> DNGGYVPAVVIGTGYGAAVSALRLGEAGVQTLMLEMGQLWNQPGPDGNIFCGMLNPDKRSSWFKNRTEAPLGSFLWLDVVNRNIDPYAGVLDRVNYDQMSVYVGRGVGGGSLVNGGMAVEPKRSYFEEILPRVDSSEMYDRYFPRANSMLRVNHIDTKWFEDTEWYKFARVSREQAGKAGLGTVFVPNVYDFGYMQREAAGEVPKSALATEVIYGNNHGKQSLDKTYLAAALGTGKVTIQTLHQVKTIRQTKDGGYALTVEQKDTDGKLLATKEISCRYLFLGAGSLGSTELLVRARDTGTLPNLNSEVGAGWGPNGNIMTARANHMWNPTGAHQSSIPALGIDAWDNSDSSVFAEIAPMPAGLETWVSLYLAITKNPQRGTFVYDAATDRAKLNWTRDQNAPAVNAAKALFD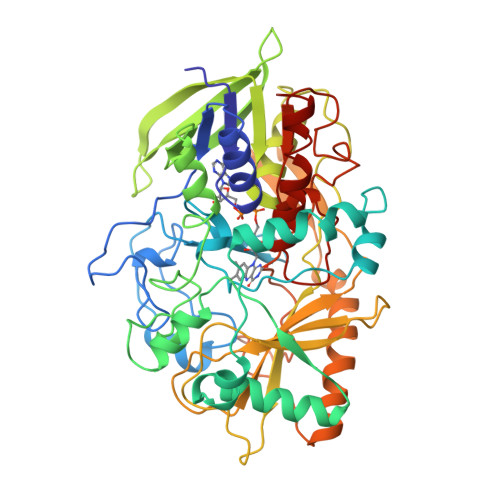RINKANGTIYRYDLFGTQLKAFADDFCYNPLGGCVLGKATDDYGRVAGYKNLYVTDGSLIPGSVGVNPFVTITALAERNVERIIKQDVTAS>[3x]MSGRVGDLSPRQKEALAKFRENVQDVLPALPNPDDYFLLRWLRARSFDLQKSEAMLRKHVEFRKQKDIDNIISWQPPEVIQQYLSGGMCGYDLDGCPVWYDIIGPLDAKGLLFSASKQDLLRTKMRECELLLQECAHQTTKLGRKVETITIIYDCEGLGLKHLWKPAVEAYGEFLC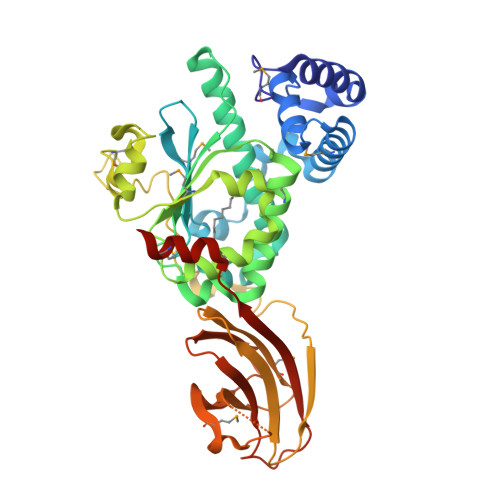MFEENYPETLKRLFVVKAPKLFPVAYNLIKPFLSEDTRKKIMVLGANWKEVLLKHISPDQVPVEYGGTMTDPDGNPKCKSKINYGGDIPRKYYVRDQVKQQYEHSVQISRGSSHQVEYEILFPGCVLRWQFMSDGADVGFGIFLKTKMGERQRAGEMTEVLPNQRYNSHLVPEDGTLTCSDPGIYVLRFDNTYSFIHAKKVNFTVEVLLPDKASEEKMKQLGAGTPK> MRGSHHHHHHGSMSQPDATPFDYILSGGTVIDGTNAPGRLADVGVRGDRIAAVGDLSASSARRRIDVAGKVVSPGFIDSHTHDDNYLLKHRDMTPKISQGVTTVVTGNCGISLAPLAHANPPAPLDLLDEGGSFRFARFSDYLEALRAAPPAVNAACMVGHSTLRAAVMPDLRREATADEIQAMQALADDALASGAIGISTGAFYPPAAHASTEEIIEVCRPLITHGGVYATHMRDEG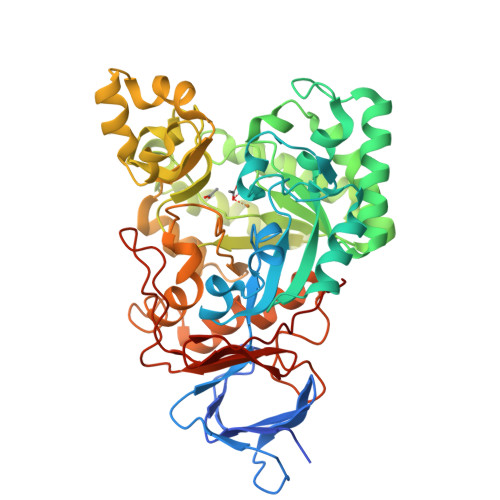EHIVQALEETFRIGRELDVPVVISHHKVMGKLNFGRSKETLALIEAAMASQDVSLDAYPYVAGSTMLKQDRVLLAGRTLITWCKPYPELSGRDLEEIAAERGKSKYDVVPELQPAGAIYFMMDEPDVQRILAFGPTMIGSDGLPHDERPHPRLWGTFPRVLGHYSRDLGLFPLETAVWKMTGLTAAKFGLAERGQVQPGYYADLVVFDPATVADSATFEHPTERAAGIHSVYVNGAAVWEDQSFTGQHAGRVLNRAGA>MERAESSSTEPAKAIKPIDRKSVHQICSGQVVLSLSTAVKELVENSLDAG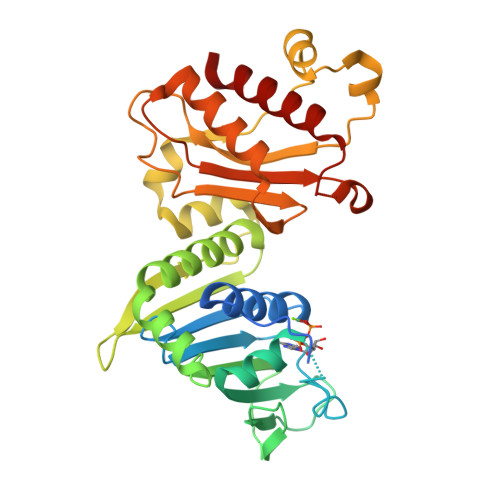ATNIDLKLKDYGVDLIEVSDNGCGVEEENFEGLTLKHHTSKIQEFADLTQVETFGFRGEALSSLCALSDVTISTCHASAKVGTRLMFDHNGKIIQKTPYPRPRGTTVSVQQLFSTLPVRHKEFQRNIKKEYAKMVQVLHAYCIISAGIRVSCTNQLGQGKRQPVVCTGGSPSIKENIGSVFGQKQLQSLIPFVQLPPSDSVCEEYGLSCSDALHNLFYISGFISQCTHGVGRSSTDRQFFFINRRPCDPAKVCRLVNEVYHMYNRHQYPFVVLNISVDSECVDINVTPDKRQILLQEEKLLLAVLKTSLIGMFD[2x]>GSKEDLPAYEEAEITKVGAYHRFYSGDKDAITGENIVAEKELDRTNNIDSEHGVA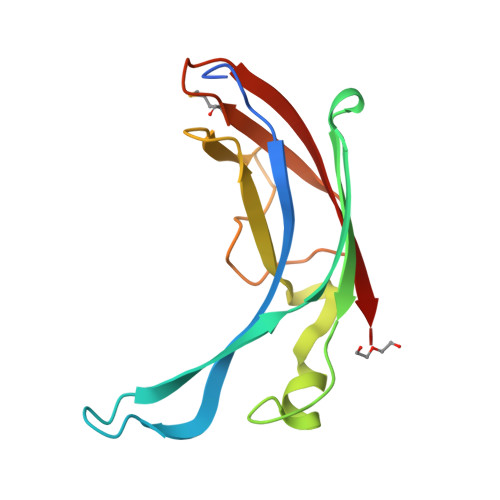TAVFTIPAAGGKFTEAERAKVSLSNLVVYVNVSTAARVTPLDGSPKFGVPADWTREHKYSVMAADGTKKIWTVKVTLNK[4x]> GSMEVLKNIRIYPLSNFITSTKNYINLPNELRNLISEEQESKLGFLHIIESDFKPSVALQKLVNCTTGDEKILIIDIVSIWSQQKQRQHGAIYMNSLSCINITGLIVFLELLYDSPMDALRRCQVDNFNFQLRGIVIDNLSFLNFESDKNYDVINLSKFEKLFKILRKLREFLGCWIITKSFPTDFYNGIENTLVDKWSIKRKSGVTLYPTKLPDSYMKGMDLIIYREVVDGRPQYRRIAALEE;> MEYEDLELITIWPSPTKNKLCQFIKQNLSKEHVVTQLFFIDATSSFPLSQFQKLVPPTLPENVRIYENIRINTCLDLEELSAITVKLLQILSMNKINAQRGTEDAVTEPLKIILYINGLEVMFRNSQFKSSPQRSHELLRDTLLKLRVMGNDENENASIRTLLEFPKEQLLDYYLKKNNNTRTSSVRSKRRRIKNGDSLAEYIWKYYAD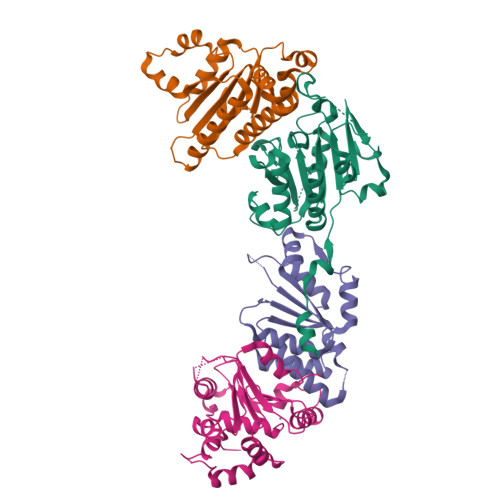SLFE;> MQFEERLQQLVESDWSLDQSSPNVLVIVLGDTARKYVELGGLKEHVTTNTVAGHVASRERVSVVFLGRVKYLYMYLTRMQAQANGPQYSNVLVYGLWDLTATQDGPQQLRLLSLVLRQCLSLPSKVEFYPEPPSSSVPARLLRFWDHIIR;> MSKDVIEYSKLFAKLVNTNDDTKLDDTIASFLYYMFPRELFIRAISLLESSDMFIYILDRVHNKEGNEHTSLIDVLVDEFYKGSSNSLLEYRLIVKDTNDGAPPILVDIAHWFCSCEEFCKYFHEALEKTDEKEELHDVLINEVDDHLQFSDDRFAQLDPHSLSKQWYFKFDKVCCSHLLAFSILLRSSINVLKFFTVNSNKVFVIAIDNIDEWLNLHINIVE> MVQELSIERLLEMESLV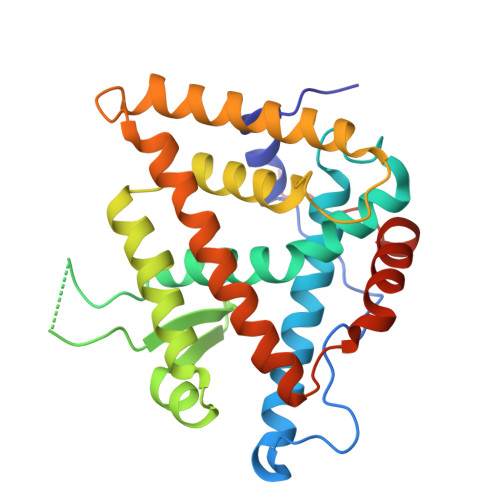ADPSEEFQFLRVGPDSNVPPKFRAPVSSLCQIGNKQIAALVVWARDIPHFSQLEMEDQILLIKGSWNELLLFAIAWRSMEFLTEERDGVDGTGNRTTSPPQLMCLMPGMTLHRNSALQAGVGQIFDRVLSELSLKMRTLRVDQAEYVALKAIILLNPDVKGLKNRQEVEVLREKMFLCLDEYCRRSRSSEEGRFAALLLRLPALRSISLKSFEHLFFFHLVADTSIAGYIRDALRNHAPPIDTNMM(2R)-3-(1H-indol-3-yl)-2-methylsulfanyl-propanoic acid | C12 H13 N 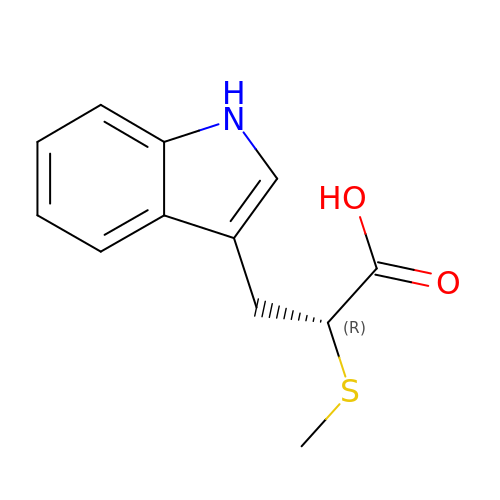O2 S | ZGMAESWNIVTLJE-LLVKDONJSA-N>NAQFLHTQVGRGLLGAVVNPLGEVTDKFAVTDNSEILYRPVDNAPPLYSE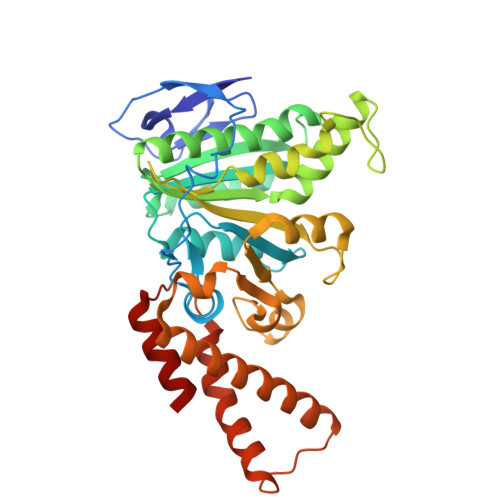RAAIEKPFLTGIKVIDSLLTCGEGQRMGIFASAGCGKTFLMNMLIEHSGADIYVIGLIGERGAEVTETVDYLKNSEKKSRCVLVYATSDYSSVDRCNAAYIATAIAEFFRTEGHKVALFIDSLTRYARALRDVALAAGESPARRGYPVSVFDSLPRLLERPGKLKAGGSITAFYTVLLEDDDFADPLAEEVRSILDGHIYLSRNLAQKGQFPAIDSLKSISRVFTQVVDEKHRIMAAAFRELLSEIEELRTIIDFGEYKPGENASQDKIYNKISVVESFLKQDYRLGFTYEQTMELIGETIR[2x]>MGTEESKQRVIQEYVPGKQVTLAHIIANPNEDIYKKLGLVLDKKDAIGILTITPSEASIIAADVATKASNVSLGFIDRFSGSVVISGDVSS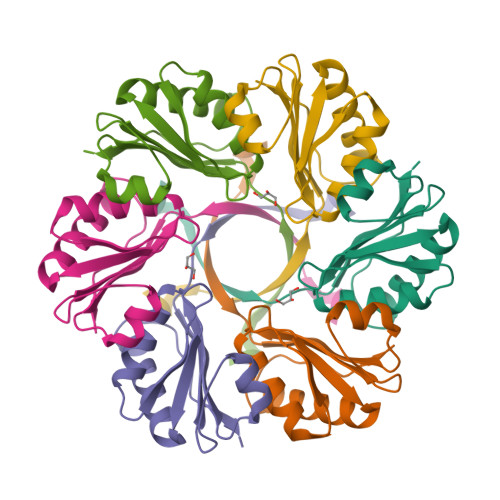VESALNDVLEVLGNMLNFSSTKITRTLEHHHHHH[2x]>[2x]MKKRLTESQFQEAIQGLEVGQQTIEIARGVL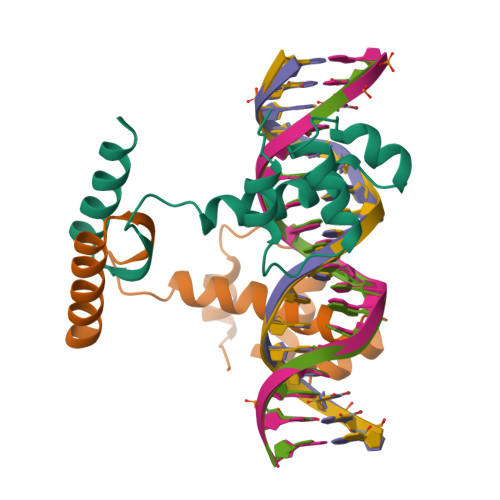VDGKPQATFATSLGLTRGAVSQAVHRVWAAFEDKNLPEGYARVTAVLPEHQAYIVRKWEADAKKKQETKR> MSNDNEVPGSMVIVAQGPDDQYAYEVPPIDSAAVAGNMFGDLIQREIYLQKNIYYPVRSIFEQGTKEKKEINKKVSDQVDGLLKQITQGKREATRQERVDVMSAVLHKMESDLEGYKKTFTKGPFIDYEKQSSLSIYEAWVKIWEKNSWEERKKYPFQQLVRDELERAVAYYKQDSLSEAVKVLRQELNKQKALKEKEDLSQLERDYRTRKANLQMKVQSELDQAGSALPPLVSPTPEQWLERATRLVTQAIADKKQLQTTNNTLIKNSPTPLEKQKAIYNGELLVDEIASLQARLVKLNAETTRRRTEAERKAA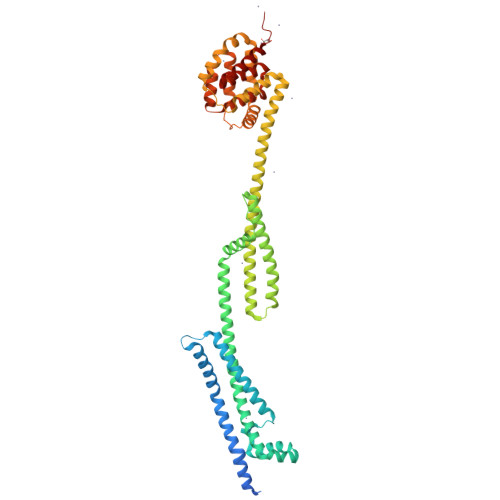EEQALQDAIKFTADFYKEVTEKFGARTSEMARQLAEGARGKNIRSSAEAIKSFEKHKDALNKKLSLKDRQAIAKAFDSLDKQMMAKSLEKFSKGFGVVGKAIDAASLYQEFKISTETGDWKPFFVKIETLAAGAAASWLVGIAFATATATPIGILGFALVMAVTGAMIDEDLLEKANNLVISILEHHHHHH>[4x]MTNQK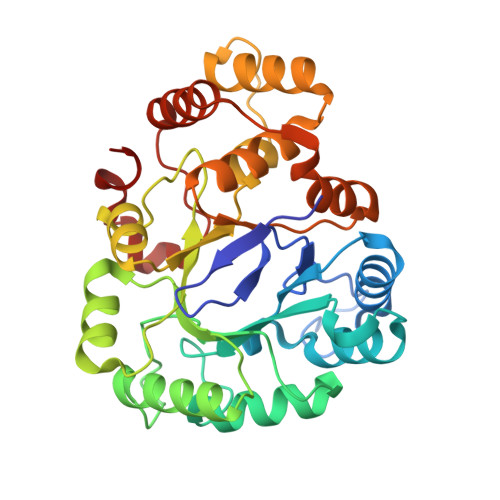FFTLSNGNKIPAVAVVGTGTKWAHAEETDATFSQELTDIVKLSLDTVPGIVHIDAAEMYKTYPELGAALKETKKPREEIFITDKFSSLHKISEDPKSALETALNKLGVDYVDLYLIHSPFFDKDLNIDLETAWKQLEELYKSGKAKNIGVSNFTVEDLKKVLAIAEIKPQVNQIEFSPFLQNQTPGIVEFSQKNDILLEAYSPLGPLAKKPTDADQQPFYQYLKELSEKYNKTEAQVLLLWVYKRGILPVTTSAKIERIKQAQDIFSFDLTEEEVKKITDLGLQHEPVRLWHVDFYTKYNSEAQK>[12x]GPELMVISRAEIYWADLGPPSGSQPAKRRPVLVI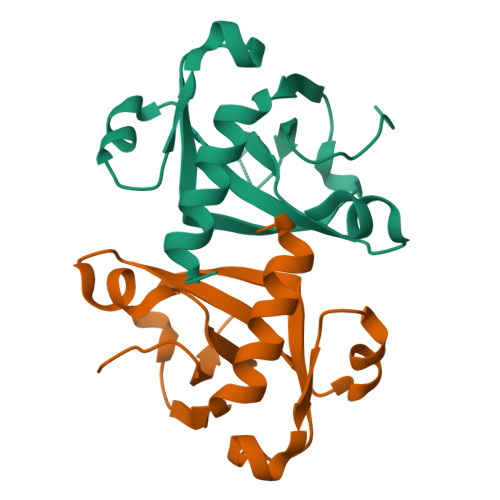QSDPYNASRLATVIAAVITSNTALAAMPGNVFLPATTTRLPRDSVVNVTAIVTLNKTDLTDRVGEVPASLMHEVDRGLRRVLDL> AATDISGAFEYSGWENFHRTQWSWDKKTRGAHLVNCTGACPHFVYSKDGVVMREEQSKDIAPMPNIPEYNPRGCNKGECGHDYMYGPHRIKYPLIRVGERGEGKWRRATWEEALDMIADKCVDTIKNHAPDCISVYSPVPAVSPVSFSAGHRFAHYIGAHAHTFYDWYGDHPTGQTQTCGVQGDTCETADWFNSKYIILWGSNPTQTRIPDAHFLSEAQLNGAKIVSISPDYNSSTIKVDKWIHPQPGTDGALAMAMAHVIIKEKLYDAHSLKEQTDLSYLVRSDTKRFLREADVVAGGSKDKFYFWNAKTGKPVIPKGSWGDQPEKKGSPVGFLGRNTFAFPKGYIDLGDLDPALEGKFNMQLLDGKTVEVRPVFEILKSRLMADNTPEKAAKITGVTAKAITELAREFATAKPSMIICGGGTQHWYYSDVLLRAMHLLTALTGTEGTNGGGMNHYIGQEKPAFVAGLVALAFPEGVNKQRFCQTTIWTYIHAEVNDEIISSDIDTEKYLRDSITTGQMPNMPEQGRDPKVFFVYRGNWLNQAKGQKYVLENLWPKLELIVDINIRMDSTALYSDVVLPSAHWYEKLDLNVTSEHSYINMTEPAIKPMWESKTDWQIFLALAKRVEMAAKRKKYEKFNDEKFKWVRDLSNLWNQMTMDG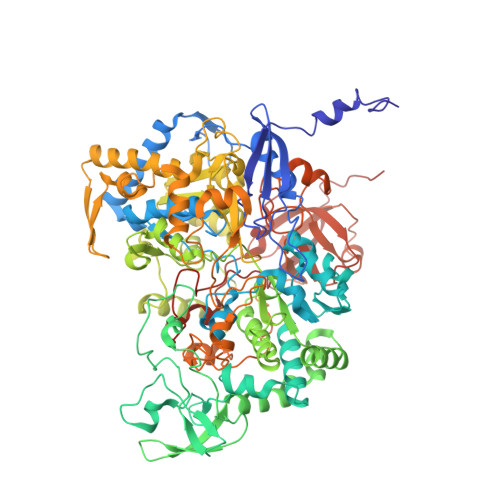KLAEDEAAAQYILDNAPQSKGITIQMLREKPQRFKSNWTSPLKEGVPYTPFQYFVVDKKPWPTLTGRQQFYLDHDTFFDMGVELPTYKAPIDADKYPFRFNSPHSRHSVHSTFKDNVLMLRLQRGGPSIEMSPLDAKPLGIKDNDWVEAWNNHGKVICRVKIRNGEQRGRVSMWHCPELYMDLLTGGSQSVCPVRINPTNLVGNYGHLFFRPNYYGPAGSQRDVRVNVKRYIGATPISF>[2x]GAMRKIGIIGGTFDPPHYGHLLIANEVYHALNLEEVWFLPNQIPPHKQGRNITSVESRLQMLE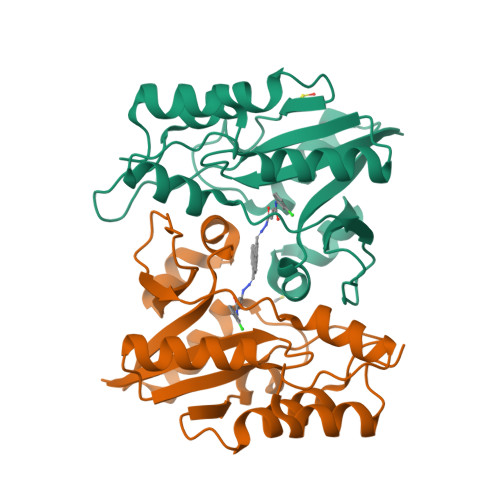LATEAEEHFSICLEELSRKGPSYTYDTMLQLTKKYPDVQFHFIIGGDMVEYLPKWYNIEALLDLVTFVGVARPGYKLRTPYPITTVEIPEFAVSSSLLRERYKEKKTCKYLLPEKVQVYIERNGLYES> MALSLYEKMLHKGMIIKNSNVYEKIKEIDTIIFEKTGTLTYGTPIVTQFIGDSLSLAYAASVEALSSHPIAKAIVKYAKEQGVKILEVKDFKEISGIGVRGKISDKIIEVKKAE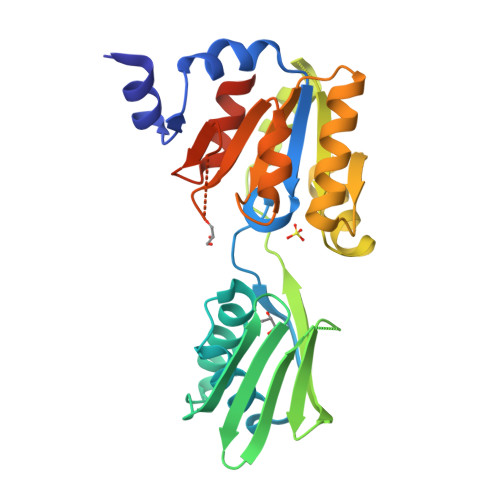NNNDIAVYINGEPIASFNISDVPRPNLKDYLEKLKNEGLKIIILSGDKEDKVKELSKELNIQEYYSNLSPEDKVRIIEKLKQNGNKVLMIGDGVNDAAALALADVSVAMGNGVDISKNVADIILVSNDIGTLLGLIKNRKRLSNAIPSN Aminoacyl-tRNA synthetases (AARSs), a family of essential protein synthesis enzymes, are attractive targets for drug development. Here we present five unusual crystal structures showing that threonyl-tRNA synthetase (ThrRS) is covalently inhibited by a natural product, obafluorin (OB). OB contains a β-lactone ring with a 2,3-dihydroxybenzamidyl moiety attached to the α position and a 4-nitrobenzyl moiety attached to the β position. When ThrRS catalyzes tRNA aminoacylation, the Zn2+ ion recognizes and binds l-threonine, assisting in the l-threonine activation reaction.

We hypothesized that if Tyr462 was mutated to a lysine residue, the mutant protein ThrRS_Y462K should also be covalently inhibited by OB, because these two residues have similar side chain lengths and lysine has stronger nucleophilicity. OB increased the Tm of ThrRS_WT by 34.8 °C, which was 2.7 °C more than that of 36j. Interestingly, OB also increased the Tm of ThrRS_Y462K by 36.8 °C, suggesting that OB forms a covalent bond with the engineered Lys462. To visualize the covalent bond, we determined the 1.9 Å structure of ThrRS_Y462K in the presence of OB. The overall structure of the ThrRS_Y462K mutant was very similar to that of the wild-type protein. As predicted, Lys462 also induced the ring-opening and covalent bond formation of the β-lactone. At the same time, coordination bonds were formed between the o-diphenol group and the Zn2+ ion, and stacking interactions were maintained between the nitrobenzene group and ThrRS Tyr313 and Arg363 residues.

> MRDHRKIGKQLDLYHMQEEAPGMVFWHNDGWTIFRELEVFVRSKLKEYQYQEVKGPFMMDRVLWEKTGHWDNYKDAMFTTSSENREYCIKPMNCPGHVQIFNQGLKSYRDLPLRMAEFGSCHRNEPSGSLHGLMRVRGFTQDDAHIFCTEEQIRDEVNGCIRLVYDMYSTFGFEKIVVKLSTRPEKRIGSDEMWDRAEADLAVALEENNIPFEYQLGEGAFKGPKIEFTLYDCLDRAWQCGTVQLDFSLPSRLSASYVGEDNERKVPVMIHRAILGSMERFIGILTEEFAGFFPTWLAPVQVVIMNITDSQSEYVNELTQKLSNAGIRVKADLRNEKIGFKIREHTLRRVPYMLVCGDKEVESGKVAVRTRRGKDLGSMDVNEVIEKLQQEIRSRSLKQLEELEHHHHHH> GIDELYKKEFGIVAGVDEAGRGCLAGPVVAAAVVLEKEIEGINDSKQLSPAKRERLLDEIMEKAAVGIGIASPEEIDLYNIFNATKLAMNRALENLSVKPSFVLVNGKGIELSVPGTCLVKGDQKSKLIGA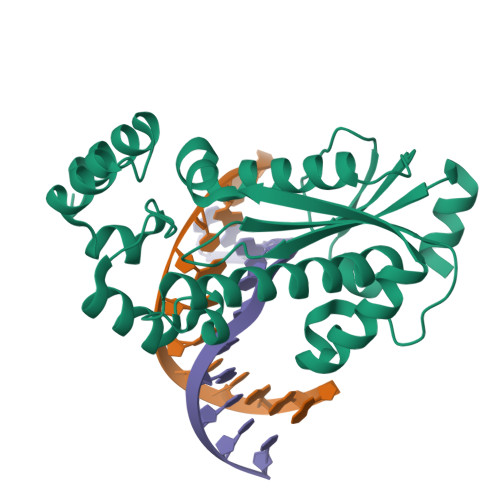ASIVAKVFRDRLMSEFHRMYPQFSFHKHKGYATKEHLNEIRKNGVLPIHRLSFEPVLELLTDDLLREFFEKGLISENRFERILNLLGARKS> MCASRDDWRCARSMHEFSAKDIDGHMVNLDKYRGFVCIVTNVASQUGKTEVNYTQLVDLHARYAECGLRILAFPCNQFGKQEPGSNEE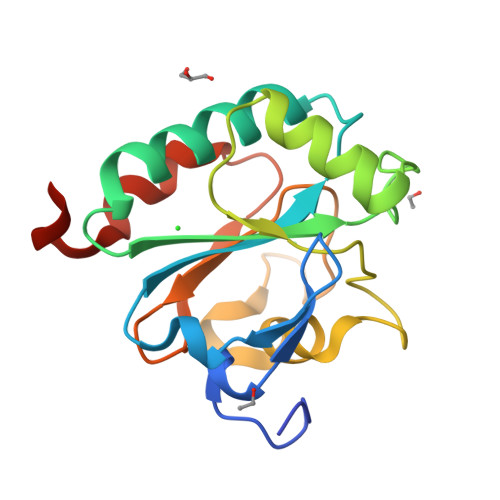IKEFAAGYNVKFDMFSKICVNGDDAHPLWKWMKIQPKGKGILGNAIKWNFTKFLIDKNGCVVKRYGPMEEPLVIEKDLPHYFHHHHHH>MTKPLDGINVLDFTHVQAGPACTQMMGFLGANVIKIERRGSGDMTRGFLQDKPNVDSLYFTMFNCNKRSIELDMKTPEGKELLEQMIKKADVMVENFGPGALDRMGFTWEYIQELNPRVILASVKGYAEGHANEHLKVYENVAQCSGGAAATTGFWDGPPTVSGAALGDSNSGMHLMIGILAALEIRHKTGRGQKVAVAMQDAVLNLVRIKLRDQQRLERT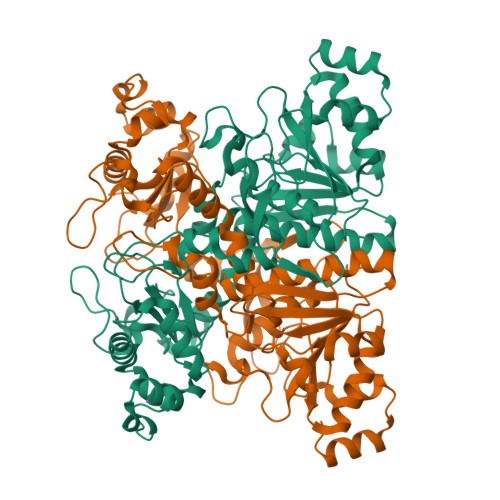GILAEYPQAQPNFAFDRDGNPLSFDNITSVPRGGNAGGGGQPGWMLKCKGWETDADSYVYFTIAANMWPQICDMIDKPEWKDDPAYNTFEGRVDKLMDIFSFIETKFADKDKFEVTEWAAQYGIPCGPVMSMKELAHDPSLQKVGTVVEVVDEIRGNHLTVGAPFKFSGFQPEITRAPLLGEHTDEVLKELGLDDAKIKELHAKQVV[2x]> MFGSGNVLPVKIQPPLLRPLAYRVLSRKYGLSIKSDGLSALAEFVGTNIGANWR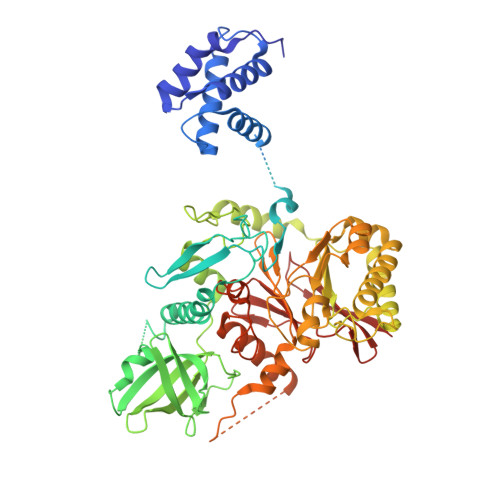QGPATIKFLEQFAAVWKQQERGLFIDQSGVKEVIQEMKEREKVEWSHEHPIQHEENILGRTDDDENNSDDEMPIAADSSLQNVSLSSPMRQPTERDEYKQPFKPESSKALDWRDYFKVINASQQQRFSYNPHKMQFIFVPNKKQNGLGGIAGFLPDIEDKVQMFLTRYYLTNDRVMRNENFQNSDMFNPLSSMVSLQNELSNTNRQQQSSSMSITPIKNLLGRDAQNFLLLGLLNKNFKGNWSLEDPSGSVEIDISQTIPTQGHYYVPGCMVLVEGIYYSVGNKFHVTSMTLPPGERREITLETIGNLDLLGIHGISNNNFIARLDKDLKIRLHLLEKELTDHKFVILGANLFLDDLKIMTALSKILQKLNDDPPTLLIWQGSFTSVPVFASMSSRNISSSTQFKNNFDALATLLSRFDNLTENTTMIFIPGPNDLWGSMVSLGASGTLPQDPIPSAFTKKINKVCKNVVWSSNPTRIAYLSQEIVIFRDDLSGRFKRHRLEFPFNESEDVYTENDNMMSKDTDIVPIDELVKEPDQLPQKVQETRKLVKTILDQGHLSPFLDSLRPISWDLDHTLTLCPIPSTMVLCDTTSAQFDLTYNGCKVINPGSFIHNRRARYMEYVPSSKKTIQEEIYI> MDGMFA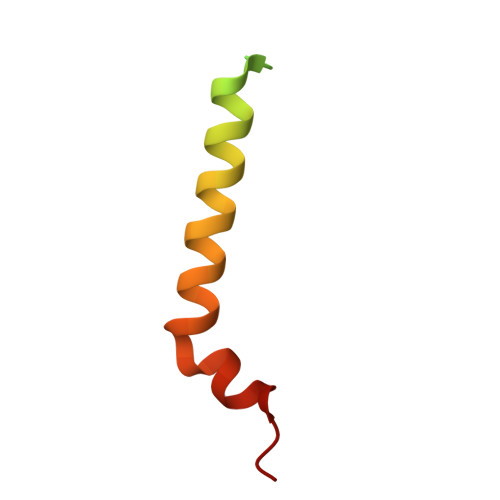MPGAAAGAASPQQPKSRFQAFKESPLYTIALNGAFFVAGVAFIQSPLMDMLAPQL>MERLRQIASQATAASAAPARPAHPLDPLSTAEIKAATNTVKSYFAGKKISFNTVTLREPARKAYIQWKEQGGPLPPRLAYYVILEAGKPGVKEGLVDLASLSVIETRALETVQPILTVEDLCSTEEVIRNDPAVIEQCVLSGIPANEMHKVYC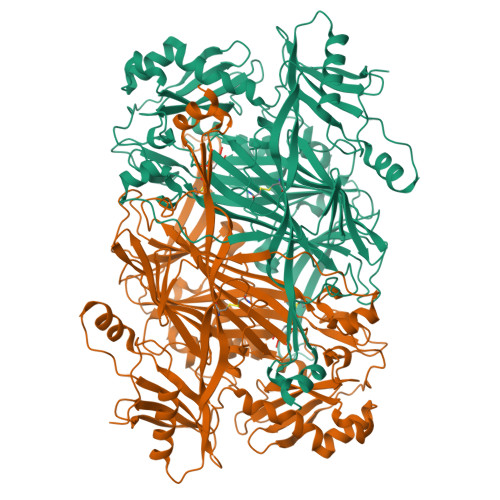DPWTIGYDERWGTGKRLQQALVYYRSDEDDSQYSHPLDFCPIVDTEEKKVIFIDIPNRRRKVSKHKHANFYPKHMIEKVGAMRPEAPPINVTQPEGVSFKMTGNVMEWSNFKFHIGFNYREGIVLSDVSYNDHGNVRPIFHRISLSEMIVPFGSPEFPHQRKHALDIGEYGAGYMTNPLSLGCDCKGVIHYLDAHFSDRAGDPITVKNAVCIHEEDDGLLFKHSDFRDNFATSLVTRATKLVVSQIFTAANXEYCLYWVFMQDGAIRLDIRLTGILNTYILGDDEEAGPWGTRVYPNVNAHNHQHLFSLRIDPRIDGDGNSAAACDAKSSPYPLGSPENMYGNAFYSEKTTFKTVKDSLTNYESATGRSWDIFNPNKVNPYSGKPPSYKLVSTQCPPLLAKEGSLVAKRAPWASHSVNVVPYKDNRLYPSGDHVPQWSGDGVRGMREWIGDGSENIDNTDILFFHTFGITHFPAPEDFPLXPAEPITLMLRPRHFFTENPGLDIQPSYAMTTSEAKRAVHKETKDKTSRLAFEGSCCGK[6x]3,5 DIBROMOTYROSINE | C9 H9 Br2 N O3 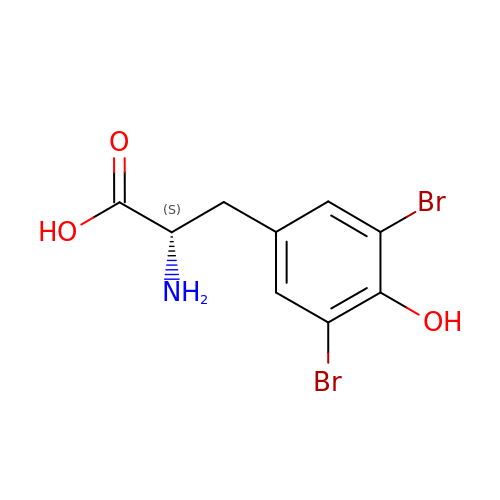| COESHZUDRKCEPA-ZETCQYMHSA-N>[2x]MIKLYGAPQSRASIIQWYLEELSLPYEFVNVNLKEGEHRQAPYLAINPFGKVPAIADGNFHLWESGAILLYLAEKASTIPADAQARALVNQW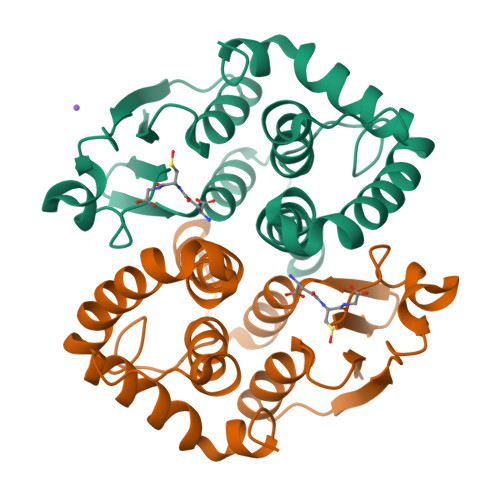ILFANSTLANGLFIEAVREKEMPRLLQSLEKILGRSPFILGEKFSVVDVAVGSILAYVPIMLKLNFDDYPAVAAYVQGLVQRPAFQASIGARLEHHHHHH> ESQPDPKPDELHKSSKFTGLMENMKVLYDDNHVSAINVKSIDQFLYFDLIYSIKDTKLGNYDNVRVEFKNKDLADKYKDKYVDVFGANYYYQCYFSKKTNDINSHQTDKRKTCMYGG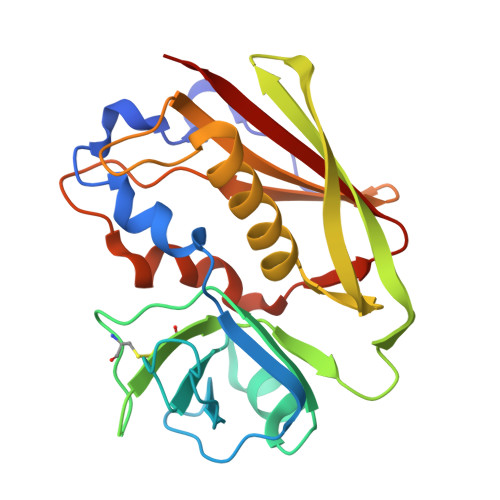VTEHNGNQLDKYRSITVRVFEDGKNLLSFDVQTNKKKVTAQELDYLTRHYLVKNKKLYEFNNSPYETGYIKFIENENSFWYDMMPAPGDKFDQSKYLMMYNDNKMVDSKDVKIEVYLTTKKK> RQEVENALDAERERAQITLASIGDGVITADTQGGISYLNPAAEQMTNWTLDKARGLPLASLFRIVDESSREEGMLLIEQILSGEIDGGREHSKLVLRHDGSSVPVTLVGAPIHRGAEITGVVLVLHDMTRERQYMARLSWQATHDALTGLTNRREFEYRLQIALERLERNSGRHALMFLDLDQFKLVNDTCGHAAGDELLRQVCTLLQQGLREGDTLARLGGDEFGILLENCPAEKAVEIADHLRKTIQDLHFTWSGQPFNCTVSVGLVHLLPGISTLEEALRSADMACYMAKEKGRNRVQVFHQDDVELSMRFGEMTWVQRIHLALEEDRFSLYAQPIVPLGEGAEEGLHVELLLRLRDEGGRLVPPLSFIPAAERYGLMTLIDRWVVENAFRTLVERAQDPRAEPIGTCAINLSGATIGDESF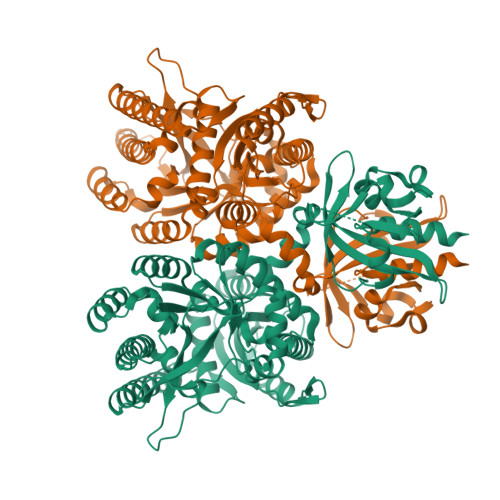LQFLTELFARYRIPPQTICFEVTETVAVANLASAIRFINELKDTGCRFSLDDFCAGMSSFIYLKHLPVDYLKIDGSFVKDMLEDPIDRAMVQVINHIGHVMGKRTIAEFVETVEVMEALREIGIDYAQGLAIGAPLPFSRQPP> MAGLSFDNYQRN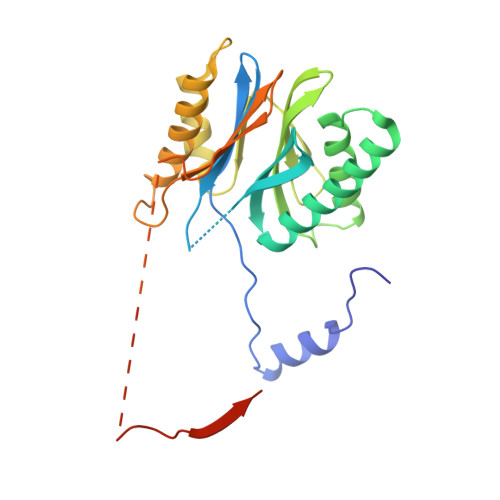NFLAENSHTQPKATSTGTTIVGVKFNNGVVIAADTRSTQGPIVADKNCAKLHRISPKIWCAGAGTAADTEAVTQLIGSNIELHSLYTSREPRVVSALQMLKQHLFKYQGHIGAYLIVAGVDPTGSHLFSIHAHGSTDVGYYLSLGSGSLAAMAVLESHWKQDLTKEEAIKLASDAIQAGIWNDLGSGSNVDVCVMEIGKDAEYLRNYLTPNVREEKQKSYKFPRGTTAVLKESIVNICDIQEEQVDITA>[3x]KTSDANETEDHLESLICKVGEKSACSLESNLEGLAGVLEADLPNYKSKILRLLCTVARLLPEKLTIYTTLVGLLNARNYNFGGEFVEAMIRQLKESLKANNYNEAVYLVRFLSDLVNCHVIAAPSMVAMFENFVSVTQEEDVPQVRRDWYVYAFLSSLPWVGKELYEKKDAEMDRIFANTESYLKRRQKTH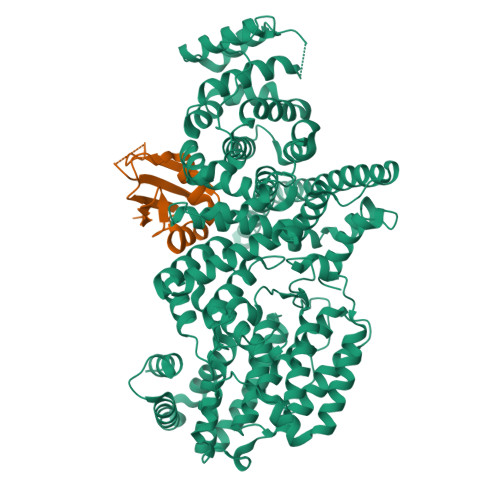VPMLQVWTADKPHPQEEYLDCLWAQIQKLKKDRWQERHILRPYLAFDSILCEALQHNLPPFTPPPHTEDSVYPMPRVIFRMFDYTDDPEGPVMPGSHSVERFVIEENLHCIIKSHWKERKTCAAQLVSYPGKNKIPLNYHIVEVIFAELFQLPAPPHIDVMYTTLLIELCKLQPGSLPQVLAQATEMLYMRLDTMNTTCVDRFINWFSHHLSNFQFRWSWEDWSDCLSQDPESPKPKFVREVLEKCMRLSYHQRILDIVPPTFSALCPSNPTCIYKYGDESSNSLPGHSVALCLAVAFKSKATNDEIFSILKDVPNPNQDDDDDEGFSFNPLKIEVFVQTLLHLAAKSFSHSFSALAKFHEVFKTLAESDEGKLHVLRVMFEVWRNHPQMIAVLVDKMIRTQIVDCAAVANWIFSSELSRDFTRLFVWEILHSTIRKMNKHVLKIQKELEEAKEKLARQHDGVLEEQIERLQEKVESAQSEQKNLFLVIFQRFIMILTEHLVRCETDGTSVLTPWYKNCIERLQQIFLQHHQIIQQYMVTLENLLFTAELDPHILAVFQQFCALQA;>[3x]DQHFRGDNEEQEKLLKKSCTLYVGNLSFYTTEEQIYELFSKSGDIKKIIMGLDKMKTACGFCFVEYYSRADAENAMRYINGTRLDDRIIRTDWDAGFK>GGAUGAAAAAACACGAUUCGGUUGGUAGUCCGGAUGCCGAAAGGUCAGUAACCUUCCACGAAAG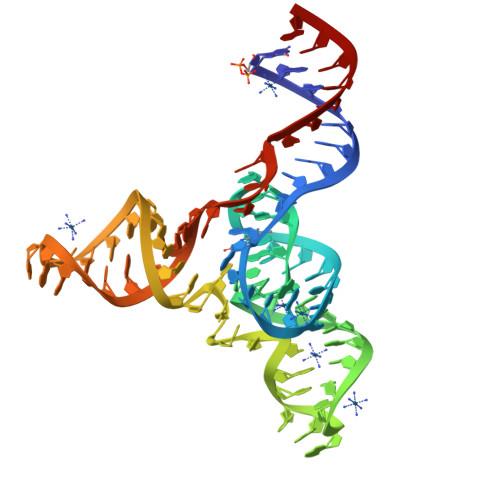UGGAUGUCCAUCAUCCA[2x]>[2x]MSMSGSNKPSVSVLGLGAMGSVLARTLLQAGYGVTVWNRSPERATALVQEGASLAREASEAINASNLIIICMIDKAVFQDVLSSLDPLLNMSGKTIVNMSTGTVDDVERIAKRVDQHNGLYVDAGIMCYPKDIGGQHTTILYSGNSDAYHAHESTLKVLAGNPKFLGADPTACTPTYLAL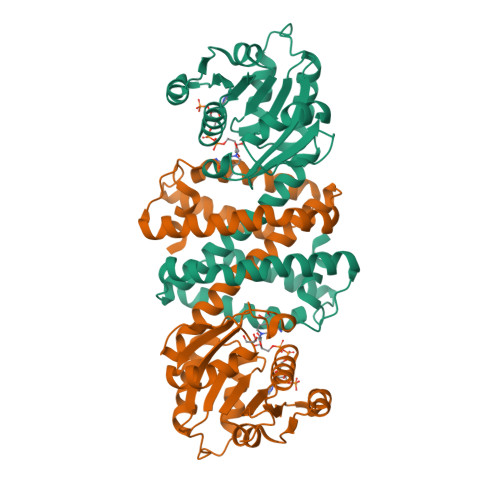YAFYFGAFAAWLEGAVLASCAGVSVQDFKALSPIMSDMLVDGIKTAADRIAASDYSGEQASVDVHVAGQEVVLDALQRANAPHASTDAYLSYCRMAQTAGMGELDIASLFKAMHP> MVSTAPYGAWQSPIDAALVASRSGRPACVGAVGDEVWWVAPRPAEAGRATLVRRRADGAEESALPAPWNVRNRVFEYSGFPWAGVPRPAGGPLLVFTHFGDQRLYAFEPDAPGGAVPRPLTPVSAVGGGLRWADPVLLPERGEVWCMAEEFTGEGPSDVRRFLAAVPLDGSAAADRSAVRELSDDAHRFVTGPRLSPDGRQAVWLAWDHPRMPWEGTELKTARVTEDGRFADTRTLLGGPEEAIAQAEWAPDGSLIVATDRTGWWNLHRVDPATGAATQLCRREEEFAGPLWTPGMRWFAPLANGLIAVVHGKGAAVLGILDPESGELVDAAGPWTEWAATLTVSGTRAVGVAASPRTAYEVVELDTVTGRARTIGARHTDPVDPAYYPEPQIRTFTAPDGREIHAHIYPPHSPDFTGPADELPPYVVMAHGGPTSRVPAVLDLDVAYFTSRGIGVADVNYGGSTG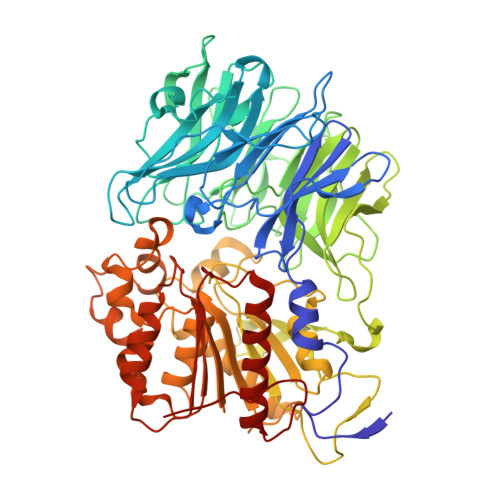YGRAYRERLRGRWGVVDVEDCAAVATALAEEGTADRARLAVRGGAAGGWTAASSLVSTDVYACGTVLYPVLDLLGWADGGTHDFESRYLDFLIGSFEEFPERYRDRAPLTRADRVRVPFLLLQGLEDPVCPPEQCDRFLEAVAGCGVPHAYLSFEGEGHGFRRKETMVRALEAELSLYAQVFGVEVAGVPLLKLGE> MTFSVDKVRADFPVLSREVNGLPLAYLDSAASAQKPSQVID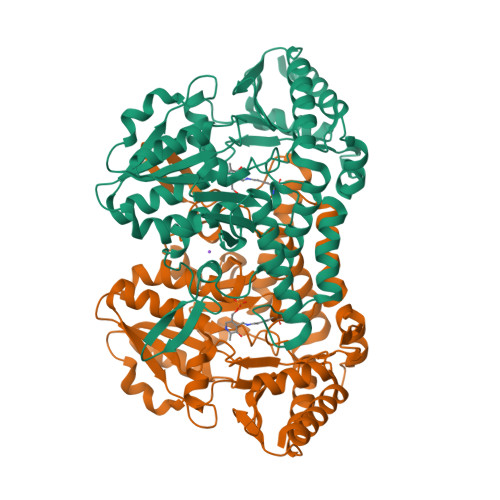AEAEFYRHGYAAVHRGIHTLSAQATEKMENVRKRASLFINARSAEELVFVRGTTEGINLVANSWGNSNVRAGDNIIISQMEHHANIVPWQMLCARVGAELRVIPLNPDGTLQLETLPTLFDEKTRLLAITHVSNVLGTENPLAEMITLAHQHGAKVLVDGAQAVMHHPVDVQALDCDFYVFSGHKLYGPTGIGILYVKEALLQEMPPWEGGGSMIATVSLSEGTTWTKAPWRFEAGTPNTGGIIGLGAALEYVSALGLNNIAEYEQNLMHYALSQLESVPDLTLYGPQNRLGVIAFNLGKHHAYDVGSFLDNYGIAVRTGHHCAMPLMAYYNVPAMCRASLAMYNTHEEVDRLVTGLQRIHRLLG>GPMVLQAQEIMTQNVVTIRGSATVADAVKLMKEKKLRGLIVEPRHEQDPYGIVTETDIVYKVAAFGHDPKTMRVYEIMAKPCVVVNPELGVEYVARLFAQTRIRRAPVIQGKTLLGIISVSDILFKSDFVEKPKRLFIEDEIEAAREDARAICAAKGETSPDCAAAWDVVEELQAEA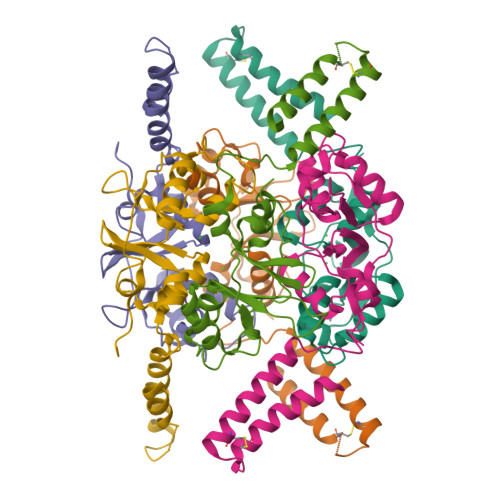SHQRAKKQGSNSFQAYCEANPDALECRIYDD[3x]>MVQPSLPQDDTPDQQEQRNRAIAQQREAYQYSETAGILLIKTLPQSEMFSLKYLIERDKGLVSLIANTLASNIENIFDPFDKLEDFEEMFPLLPKPLVMNTFRNDRVFARQRIAGPNPMVIERVVDKLPDNFPVTDAMFQKIMFTKKTLAEAIAQGKLFITNYKGLAELSPGRYEYQKNGTLVQKTKTIAAPLVLYAWKPEGFGDYRGSLAPIAIQINQQPDPITNPIYTPRDGKHWFIAKIFAQMADGNCHEAISHLARTHLILEPFVLATANELAPNHPLSVLLKPHFQFTLAINELAREQVISAGGYADDLLAGTLEASIAVIKAAIKEYMDNFTEFALPRELARRGVGIGDVDQRGENFLPDYPYRDDAMLLWNAIEVYVRDYLSLYYQSPVQIRQDTELQNWVRRLVSPEGGRVTGLVSNGELNTIEALVAIATQVIF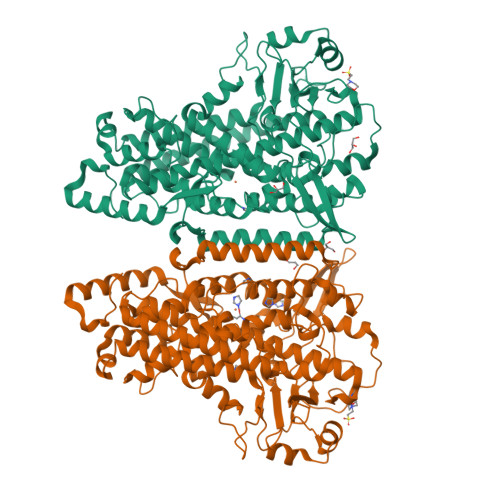VSGPQHAAVNYPQYDYMAFIPNMPLATYATPPNKESNISEATILNILPPQKLAARQLELMRTLCVFYPNRLGYPDTEFVDVRAQQVLHQFQERLQEIEQRIVLCNEKRLEPYTYLLPSNVPNSTSI[2x]>PAAMFIVNTNVPRASVPDGFLSELTQQLAQATGKPPQYIAVHVVPDQLMAFGGSSEPCALCSLHSIGKIGGAQNRSYSKLLCGLLAERLRISPDRVYINYYDMNAANVGWNNSTFA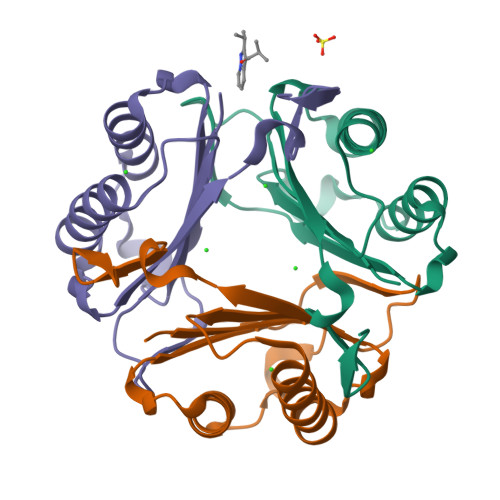[3x]3H-IMIDAZO[2,1-I]PURINE 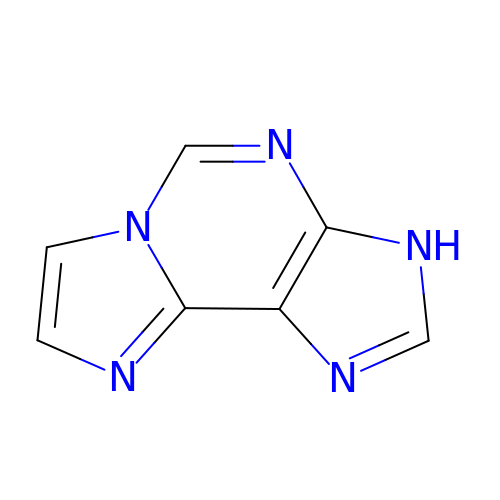| C7 H5 N5 | OGVOXGPIHFKUGM-UHFFFAOYSA-N> MRGSHHHHHHTDPQGDAAQKTDTSHHDQDHPTFNKITPNLAEFAFSLYRQLAHQSNSTNIFFSPVSIATAFAMLSLGTKADTHDEILEGLNFNLTEIPEAQIHEGFQELLRTLNQPDSQLQLTTGNGLFLSEGLKLVDKFLEDVKKLYH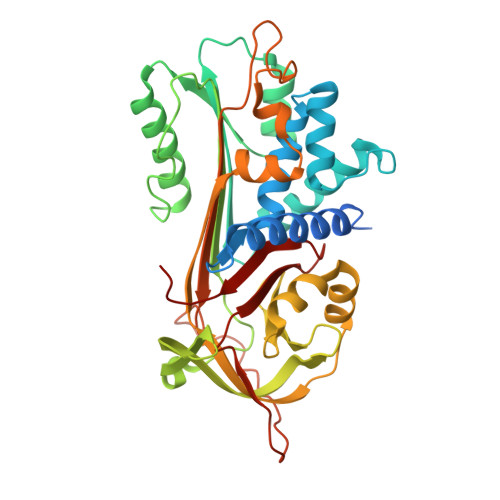SEAFTVNFGDTEEAKKQINDYVEKGTQGKIVDLVKELDRDTVFALVNYIFFKGKWERPFEVKDTEEEDFHVDQVTTVKVPMMKRLGMFNIQHCKKLSSWVLLMKYLGNATMIFFLPDEGKLQHLENELTHDIITKFLENEDRRSASLHLPKLSITGTYDLKSVLGQLGITKVFSNGADLSGVTEEAPLKLSKAVHKAVLTIDEKGTEAAGAMFLEAIPMSIPPEVKFNKPFVFLMIEQNTKSPLFMGKVVNPTQK> HHHHHHS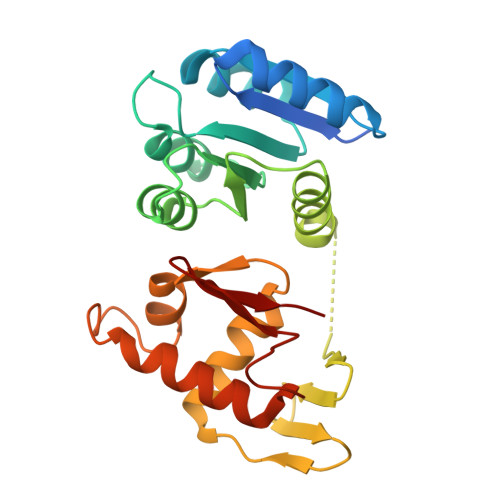SGLVPRGSHMTNVLIVEDEQAIRRFLRTALEGDGMRVFEAETLQRGLLEAATRKPDLIILDLGLPDGDGIEFIRDLRQWSAVPVIVLSARSEESDKIAALDAGADDYLSKPFGIGELQARLRVALRRHSATTAPDPLVKFSDVTVDLAARVIHRGEEEVHLTPIEFRLLAVLLNNAGKVLTQRQLLNQVWGPNAVEHSHYLRIYMGHLRQKLEQDPARPRHFITETGIGYRFML>[2x]SATETQIRIGVMGCADIA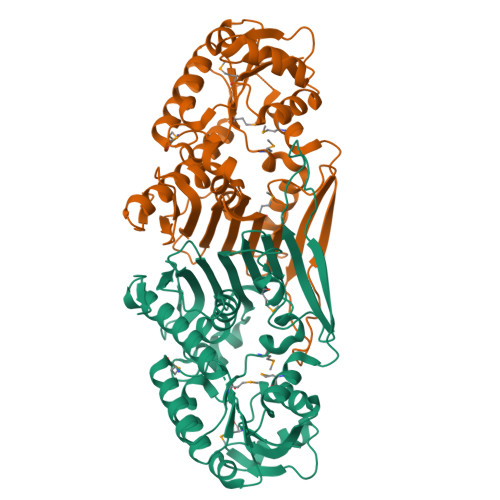RKVSRAIHLAPNATISGVASRSLEKAKAFATANNYPESTKIHGSYESLLEDPEIDALYVPLPTSLHVEWAIKAAEKGKHILLEKPVAMNVTEFDKIVDACEANGVQIMDGTMWVHNPRTALLKEFLSDSERFGQLKTVQSCFSFAGDEDFLKNDIRVKPGLDGLGALGDAGWYAIRATLLANNFELPKTVTAFPGAVLNEAGVILSCGASLSWEDGRTATIYCSFLANLTMEITAIGTKGTLRVHDFIIPYKETEASFTTSTKAWFNDLVTAWVSPPSEHTVKTELPQEACMVREFARLVGEIKNNGAKPDGYWPSISRKTQLVVDAVKESVDKNYQQISLSGR>[2x]UUGC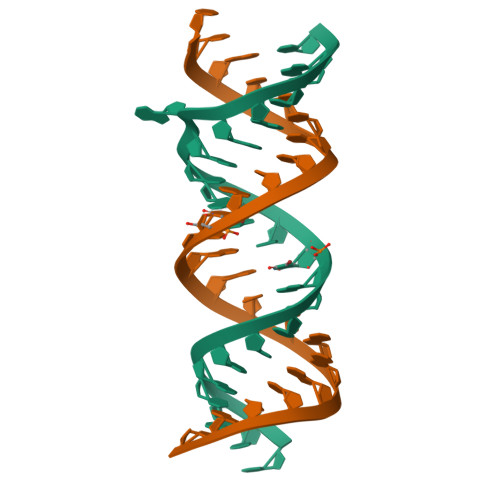GUCCCGUCGACGAAGUCGC>VGPKTGEENQVLVPNLNPTPENLEVVGDGFKITSSINLVGEEEADENAVNALREFLTANNIEINSENDPNSTTLIIGEVDDDIPELDEALNGTTAENLKEEGYALVSNDGKIAIEGKDGDGTFYGVQTFKQLVKESNIPEVNITDYPTVSARGIVEGFYGTPWTHQDRLDQIKFYGENKLNTYIYAPKDDPYHREKWREPYPESEMQRMQELINASAENKVDFVFGISPGIDIRFDGDAGEEDFNHLITKAESLYDMGVRSFAIYWDDIQDKSAAKHAQVLNRFNEEFVKAKGDVKPLITVPTEYDTGAMVSNGQPRAYTRIFAETVDPSIEVMWTGPGVVTNEIPLSDAQLISGIYNRNMAVWWNYPVTDYFKGKLALGPMHGLDKGLNQYVDFFTVNPMEHAELSKISIHTAADYSWNMDNYDYDKAWNRAIDMLYGDLAEDMKVFANHSTRMDNKTWAKSGREDAPELRAKMDELWNKLSSKEDASALIEELYGEFARMEEACNNLKANLPEVALEECSRQLDELITLAQGDKASLDMIVAQLNEDTEAYESAKEIAQNKLNTALSSFAVISEKVAQSFIQEALSFDLTLI[2x]

Protein O-GlcNAcylation was discovered two decades ago, and is an abundant, dynamic, and inducible posttranslational modification of serine/threonine residues on intracellular proteins in higher eukaryotes (Zachara and Hart, 2006; Hart et al., 2007). The O-GlcNAcase (OGA) hydrolyzes O-GlcNAcylated proteins to the free protein and GlcNAc (Gao et al., 2001; Hart et al., 2007). CpOGA contains an active site that is nearly identical to that of hOGA (Rao et al., 2006).

Using X-ray crystallography, enzymology, and cell biological studies on an insulinoma cell line, we show that, whereas streptozotocin competitively inhibits O-GlcNAcase and induces apoptosis, its galacto-configured derivative no longer inhibits O-GlcNAcase, yet still induces apoptosis. To further investigate the mode of inhibition of STZ, CpOGA activity was measured using the 4-methylumbelliferone-GlcNAc assay with a range of STZ concentrations and varying preincubation times of enzyme and inhibitor (2 min–18 hr). Both commercial (Sigma) and resynthesized samples showed that STZ inhibits CpOGA with an IC50 of 30 μM. However, the dose-response curves did not show an incubation time-dependent shift, suggesting STZ does not inhibit OGA through a covalent mechanism, in agreement with the structural data. Thus, in agreement with the structural data that show free, intact STZ binding to the OGA active site, there is no evidence for a time-dependent suicide/covalent inhibitory mechanism. Although our structure of the CpOGA-STZ complex does not support formation of a covalent intermediate or a tight-binding oxazolinium ion as recently suggested (Toleman et al., 2006), this complex was obtained by soaking procedures and cannot be taken as conclusive proof of the absence of such mechanisms. Nevertheless, in our hands, STZ, either resynthesized or from a commercial source, is a weak but purely competitive inhibitor without any evidence of time-dependent inhibition. Early kinetic characterization of OGA has shown that the enzyme is inhibited by GlcNAc, but not by GalNAc, unlike the GH 20 lysosomal hexosaminidases (Gao et al., 2001). This is readily explained by the structural data, which show that a conserved aspartic acid (Asp401 in CpOGA, Asp485 in hOGA) tethers the O6 and equatorial O4 hydroxyls. Indeed, mutation of Asp401 to an alanine abrogates CpOGA activity (Rao et al., 2006). Inspired by the CpOGA-STZ complex, the galacto isomer of STZ (Gal-STZ) was synthesized.> MQDADKLPHTKVTLVAPP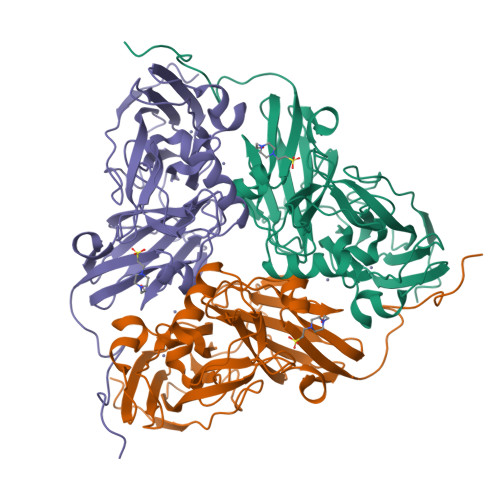QVHPHEQATKSGPKVVEFTMTIEEKKMVIDDKGTTLQAMTFNGSMPGPTLVVHEGDYVQLTLVNPATNAMPHNVDFHGATGALGGAKLTNVNPGEQATLRFKADRSGTFVYHCTPHPFMSGTLMVLPRDGLKDPQGKPLHYDRAYTIGEFDLYIPKGPDGKYKDYATLAESYGDTVQVMRTLTPSHIVFNGKVGALTGANALTAKVGETVLLIHSQANRDTRPHLIGGHGDWVWETGKFANPPQRDLETWFIRGGSAGAALYTFKQPGVYAYLNHNLIEAFELGAAGHIKVEGKWNDDLMKQIKAPAPIPR>MNPDDIVVLVGRKKSGKSYLIKHYFIPVLKAHKISYIIDDHNLLRSGSEYSKFGYNATSLSDIVSKQYVVVYDRAKNDDFFEKLWQASKLHSKKYGTT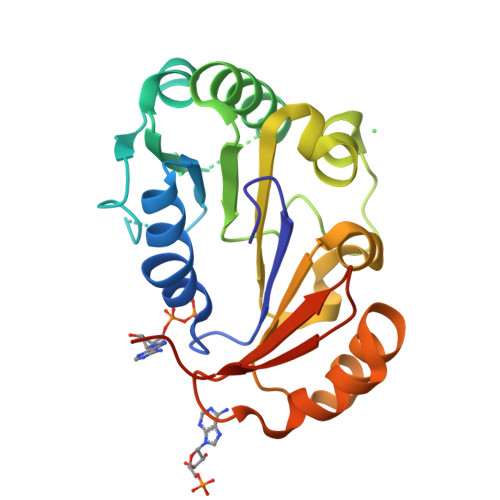VLIIDEAYYHFKYKQKVTPAIDEALHANRHAGLGLILSTQRVYDLMPIVYKQADLIIMFYTREPNELRWISKYISAEAAEKVKTLKQYHFLIYDVNSQTIKIHKPILEHHHHHH[4x]>VPRGSHMLFQNVSIAGLAHIDAPHTLTSKEINERLQPTYDRLGIKTDVLGDVAGIHARRLWDQDVQASDAATQAARKALIDANIGIEKIGLLINTSVSRDYLEPSTASIVSGNLGVSDHCMTFDVANACLAFINGMDIAARMLERGEIDYALVVDGETANLVYEKTLERMTSPDVTEEEFRNELAALTLGCGAAAMVMARSELVPDAPRYKGGVTRSATEWNKLCRGNLDRMVTDTRLLLIEGIKLAQKTFVAAKQVLGWAVEELDQFVIHQVSRPHTAAFVKSFGIDPAKVMTIFGEHGNIGPASVPIVLSKLKELGRLKKGDR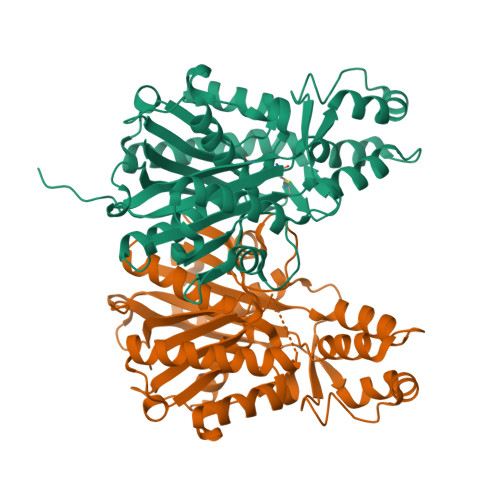IALLGIGSGLNCSMAEVVW[2x]> MTCWLRGVTATFGRPAEWPGYLSHLCGRSAAMDLGPMRKSYRGDREAFEETHLTSLDPVKQFAAWFEEAVQCPDIGEANAMCLATCTRDGKPSARMLLLKGFGKDGFRFFTNFESQKGKELDSNPFASLVFYWEPLNRQVRVEGPVKKLPEEEAECYFHSRPKSSQIGAVVSHQSSVIPDREYLR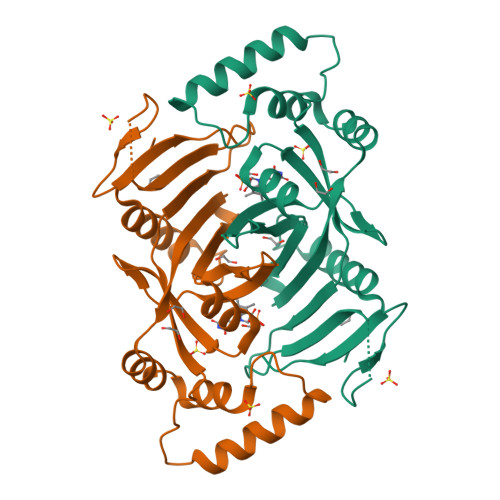KKNEELEQLYQDQEVPKPKSWGGYVLYPQVMEFWQGQTNRLHDRIVFRRGLPTGDSPLGPMTHRGEEDWLYERLAP>[2x]GHMEELNIDFDVFKKRIELLYSKYNEFEGSPNSLLFVLGSSNAENPYQKTTILHNWLLSYEFPATLIALVPGKVIIITSSAKAKHLQKAIDLFKD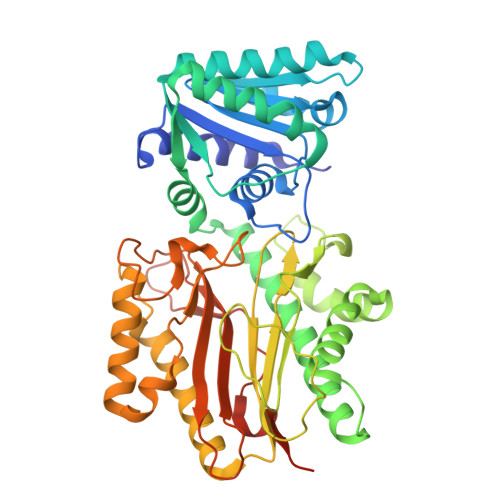PESKITLELWQRNNKEPELNKKLFDDVIALINSAGKTVGIPEKDSYQGKFMTEWNPVWEAAVKENEFNVIDISLGLSKVWEVKDVNEQAFLSVSSKGSDKFMDLLSNEMVRAVDEELKITNAKLSDKIENKIDDVKFLKQLSPDLSALCPPNYKFNFDLLDWTYSPIIQSGKKFDLRVSARSTNDQLYGNGCILASCGIRYNNYCSNITRTFLIDPSEEMANNYDFLLTLQKEIVTNILKPGRTPKEVYESVIEYIEKTKPELVPNFTKNIGSLIGLEFRDSNFILNVKNDYRKIQRGDCFNISFGFNNLKDSQSANNYALQLADTVQIPLDETEPPRFLTNYTKAKSQISFYFNNEEEDNNKKKSSPATKV> MAGAEQSQRWSLKAKTVLVTGGTKGIGHAIVEEFAGFGAVIHTCARNEYELNECLSKWQKKGFQVTGSVCDASLRPEREKLMQTVSSMFGGKLDILINNLGAIRSKPTLDY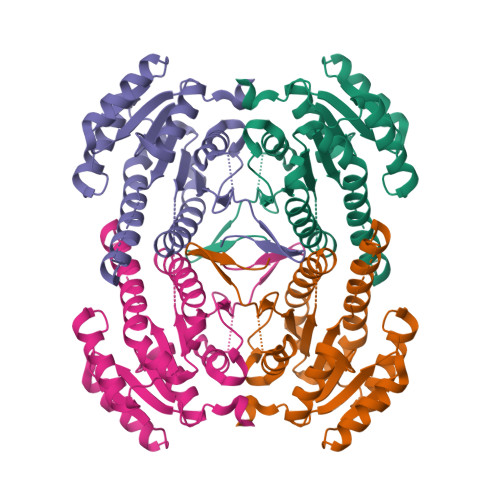TAEDFSFHISTNLESAYHLSQLAHPLLKASGCGNIIFMSSIAGVVSASVGSIYSATKGALNQLARNLACEWASDGIRANAVAPAVIATPLAEAVYDDEFKKVVISRKPLGRFGEPEEVSSLVAFLCMPAASYITGQTICVDGGLTVNGFSYQPQG> QECTKFKVSSCRECIESGPGCTWCQKLNFTGPGDPDSIRCDTRPQLLMRGCAADDIMDPTSLAETQEDHNGGQKQLSPQKVTLYLRPGQAAAFNVTFRRAKGYPIDLY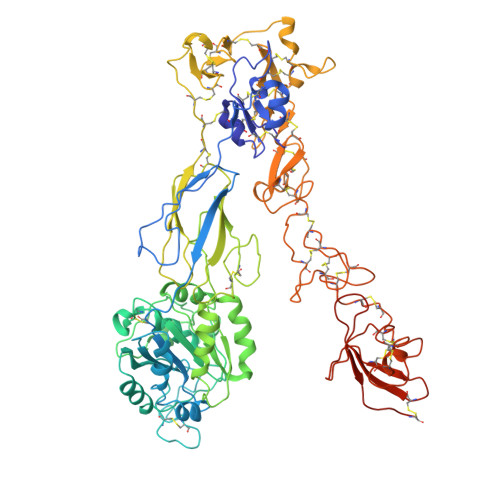YLMDLSYSMLDDLRNVKKLGGDLLRALNEITESGRIGFGSFVDKTVLPFVNTHPDKLRNPCPNKEKECQPPFAFRHVLKLTNNSNQFQTEVGKQLISGNLDAPEGGLDAMMQVAACPEEIGWRNVTRLLVFATDDGFHFAGDGKLGAILTPNDGRCHLEDNLYKRSNEFDYPSVGQLAHKLAENNIQPIFAVTSRMVKTYEKLTEIIPKSAVGELSEDSSNVVQLIKNAYNKLSSRVFLDHNALPDTLKVTYDSFCSNGVTHRNQPRGDCDGVQINVPITFQVKVTATECIQEQSFVIRALGFTDIVTVQVLPQCECRCRDQSRDRSLCHGKGFLECGICRCDTGYIGKNCECQTQGRSSQELEGSCRKDNNSIICSGLGDCVCGQCLCHTSDVPGKLIYGQYCECDTINCERYNGQVCGGPGRGLCFCGKCRCHPGFEGSACQCERTTEGCLNPRRVECSGRGRCRCNVCECHSGYQLPLCQECPGCPSPCGKYISCAECLKFEKGPFGKNCSAACPGLQLSNNPVKGRTCKERDSEGCWVAYTLEQQDGMDRYLIYVDESRECVAGPDGCGENLYFQ> LTCVKSK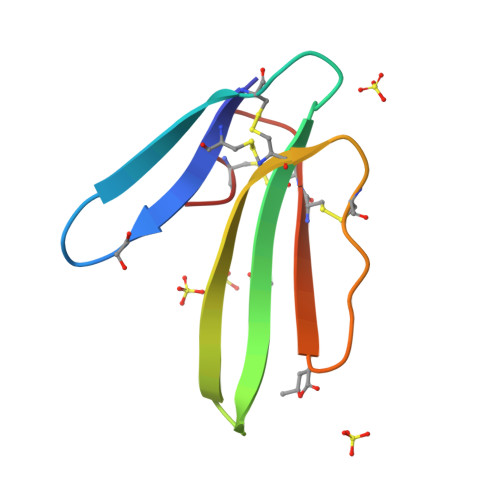SIFGVTTEDCPDGQNLCFKRRHYIVPKMYDSTRGCAATCPIAENRDVIHCCGTDKCNE> MKPTIPPDDSDTAGKQVEVEKENETIQELMIALQIHSGYTNISYTI;> MSLILDDIILSLTNANERTPPQALKTTLSLLYEKSKQYGLSSPQLQALVRLLCETSIIDTVTKVYIVENCFLPDGYLTKELLLEIINHLGTPTVFSRYRIQTPPVLQSALCKWLVHVYFLFPVHSEREHNISSSIWLHLWQFSFLQKWITPLVIWQATTPVDVKPWKLSIIKRCAMHPGYRDAPGSATLILQRFQCLVGASSQITESIITINCNRKTLKSHRNLKLDAHFLSILKRILSRAHPANENLYFQ;> MKKQDHAHIRTRKARNKELWDSLADFLKGYLVPNLDDNDESIDSLTNEVMLLMKRLIEHDLNLTLNDFSSKTIPIYRLLLRANIITVIEGSTNPGTKYIKLIDFNETSLT;> MSTPRKAAGNNENTEVSEIRTPFRERALEEQRLKDEVLIRNTPGYRKLLSASTKSHDILNKDPNEVRSFLQDLSQVLARKSQGNDTTTNKTQARNLIDELAYEESQPEENELLRSRSEKLTDNNIGNETQPDYTSLSQTVFAKLQERDKGLKSRKIDPIIIQDVPTTGHEDELTVHSPDKANSISMEVLRTSPSIGMDQVDEPPVRDPVPISITQQEEPLSEDLPSDDKEETEEAENEDYSFENTSDENLDDIGNDPIRLNVPAVRRSSIKPLQIMDLKHLTRQFLNENRIILPKQTWSTIQEESLNIMDFLKQKIGTLQKQELVDSFIDMGIINNVDDMFELAH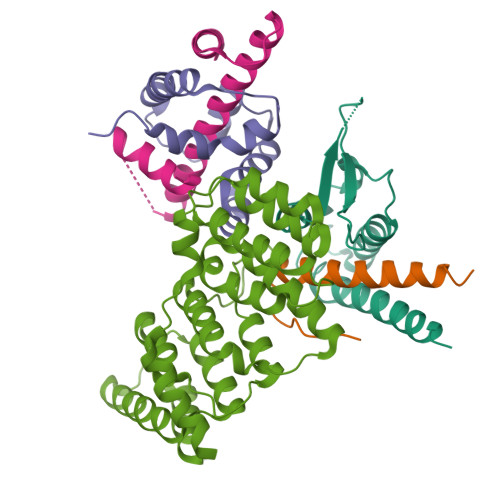ELLPLELQSRIESYLFENLYFQ;> MDTEALANYLLRQLSLDAEENKLEDLLQRQNEDQESSQEYNKKLLLACGFQAILRKILLDARTRATAEGLREVYPYHIEAATQAFLDSQ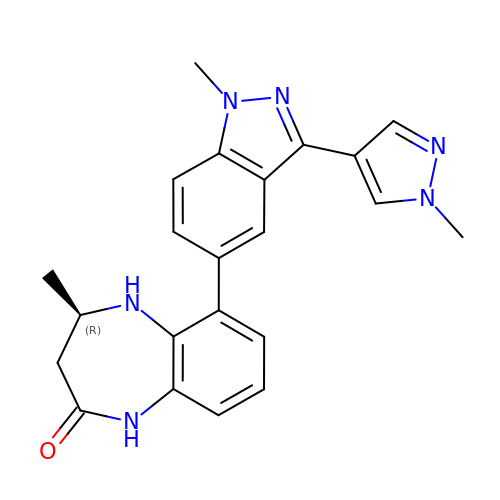(4R)-4-methyl-6-[1-methyl-3-(1-methyl-1H-pyrazol-4-yl)-1H-indazol-5-yl]-1,3,4,5-tetrahydro-2H-1,5-benzodiazepin-2-one | C22 H22 N6 O | BFTKDWYIRJGJCA-CYBMUJFWSA-N> GSDDINQKVAEQLAQKAQSSSLGYDIVESLTVEVGPRLAGSEQDKVAVDWAIAKLQSLGFDRVYKEPVTVPVWRRGIAKASILSPFPQPLVVTALGGSIATPAQGLSATIVRFDTLQDLQNAEAGSLNDKIAFIDAKTERHRDGKGYGQTASGRSRGAVAAAEKGAVGIIIRSIGTDHDRMAHTGMMRYEEGVTAIPAAAISNPDADLINAMLKRDKEVVISLELGSERRGETTSYNVIAEVKGSTKADEIVLIGAHLDSWDEGTGAIDDGAGVAIVTAAAKHILDLPQKPERTIRVVLYAAEELGLLGGKTYAKEHEAELEKHYIAAESDFGAGPIYQIDWRVADTAHSPVINAMKVAEPLGVAAGNNKASGGPDVSMLPALGV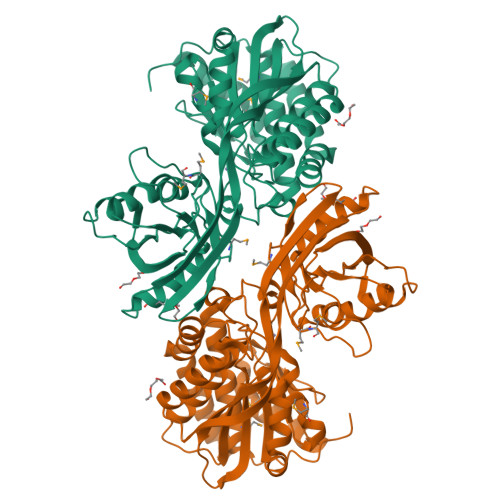PVASLRQDGSDYFDYHHTPNDTLDKINPEALAQNVAVYAQFAWVMANSKVELRPLPPKE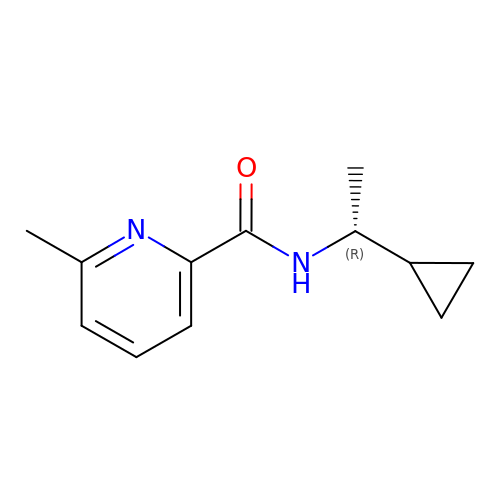(R)-N-(1-cyclopropylethyl)-6-methylpicolinamide | C12 H16 N2 O | HZPLHNFJXLSHCY-SECBINFHSA-N>PSVYDAAAQL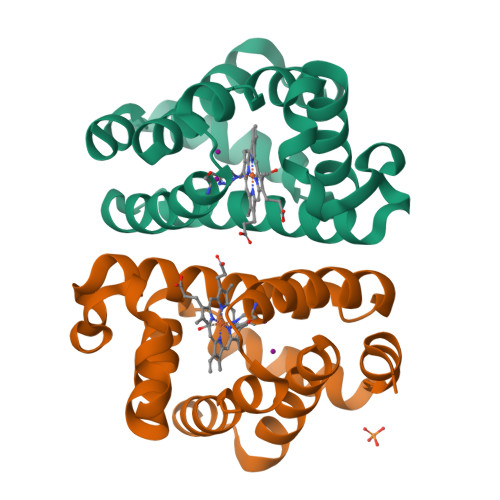TADVKKDLRDSWKVWGSDKKGNGVALMTTLFADNQETIGYFKRLGDVSQGMANDKLRGHSITLMYALQNFIDQLDNPDDLVCVVEKFAVNHITRKISAAEFGKINGPIKKVLASKNFGDKYANAWAKLVAVVQAAL[2x]8-[2-((2S)-4-HYDROXY-1-{[5-(HYDROXYMETHYL)-6-METHOXY-2-NAPHTHYL]METHYL}-6-OXOPIPERIDIN-2-YL)ETHYL]-3,7-DIMETHYL-1,2,3,7,8,8A-HEXAHYDRONAPHTHALEN-1-YL 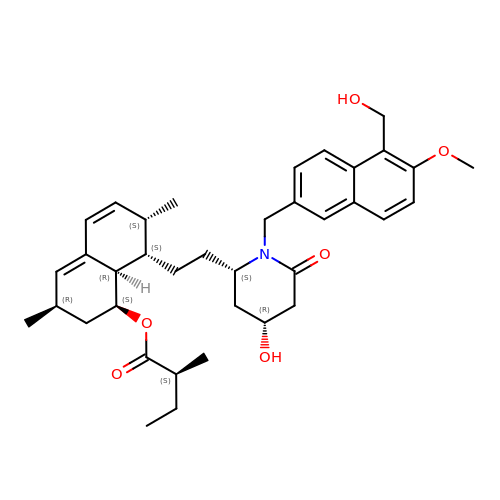2-METHYLBUTANOATE | C37 H49 N O6 | WPVRNXUYVXQXPY-YFAYRSKXSA-N> MRDHRKIGKQLDLYHMQEEAPGMVFWHNDGWTIFRELEVFVRSKLKEYQYQEVKGPFMMDRVLWEKTGHWDNYKDAMFTTSSENREYCIKPMNCPGHVQIFNQGLKSYRDLPLRMAEFGSCHRNEPSGSLHGLMRVRGFTQDDAHIFCTEEQIRDEVNGCIRLVYDMYSTFGFEKIVVKLSTRPE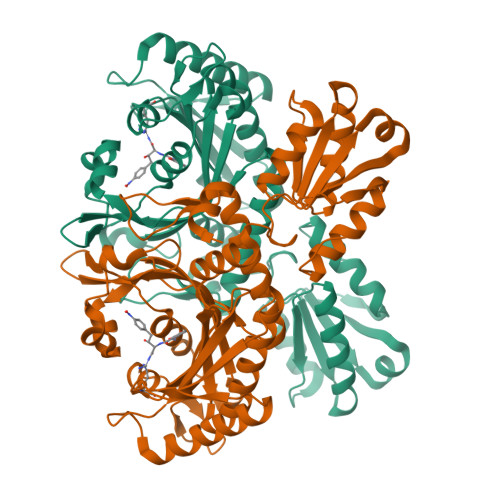KRIGSDEMWDRAEADLAVALEENNIPFEYQLGEGAFRGPKIEFTLYDCLDRAWQCGTVQLDFSLPSRLSASYVGEDNERKVPVMIHRAILGSMERFIGILTEEFAGFFPTWLAPVQVVIMNITDSQSEYVNELTQKLSNAGIRVKADLRNEKIGFKIREHTLRRVPYMLVCGDKEVESGKVAVRTRRGKDLGSMDVNEVIEKLQQEIRSRSLKQLEELEHHHHHH>[6x]MTSAEMTSPNNNSEHQAIAKMRTMIEGFDDISHGGLPIGRSTLVSGTSGTGKTLFSIQFLYNGIIEFDEPGVFVTFEETPQDIIKNARSFGWDLAKLVDE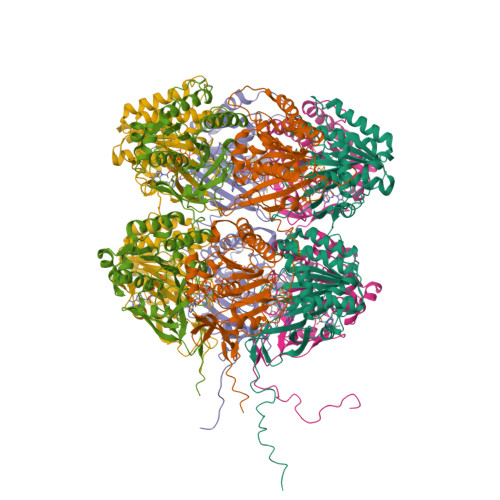GKLFILDASPDPEGQEVVGGFDLSALIERINYAIQKYRARRVSIDSVTSVFQQYDASSVVRRELFRLVARLKQIGATTVMTTERIEEYGPIARYGVEEFVSDNVVILRNVLEGERRRRTLEILKLRGTSHMKGEYPFTITDHGINIFPLGAMRLTQRSSNVRVSSGVVRLDEMCGGGFFKDSIILATGATGTGKTLLVSRFVENACANKERAILFAYEESRAQLLRNAYSWGMDFEEMERQNLLKIVCAYPESAGLEDHLQIIKSEINDFKPARIAIDSLSALARGVSNNAFRQFVIGVTGYAKQEEITGLFTNTSDQFMGAHSITDSHIAEITDTIILLQYVEIRGEMSRAINVFKMRGSWHDKAIREFMISDKGPDIKDSFRNFERIISGSPTRITVDEKSELSRIVRGVQEKGPES> MLEARLEQASLLKRVVDAIKDLVQDCNFDCNDSGIALQAMDNSHVALVSMLLKAEGFSAYRCDRNIALGINLVSLTKVLRAAQNEDILTLKADDSPDAVNLMFESAETDRISEYDIKLMDIDQEHLAIPETEYAATV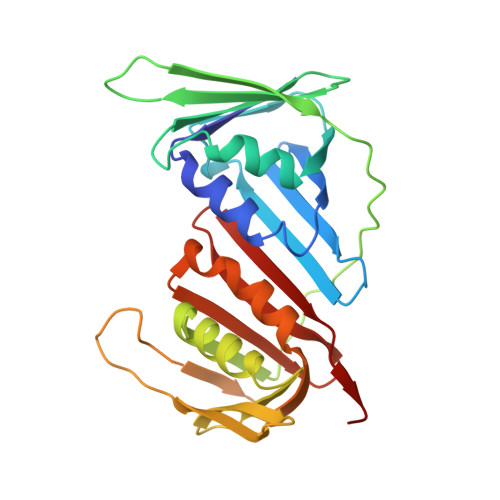EMPSAEFQRICRDLNALSESVVIEATKEGVKFSCQGDIGSGSVTIRQHTSVDKPEQNVSIALSEPVALTFSLKYLVNFCKATSLSSKVTLCLSQEVPLLVEYGLGSGHLRFYLAPKIGD>[2x]MGSSHHHHHHSSGLVPRG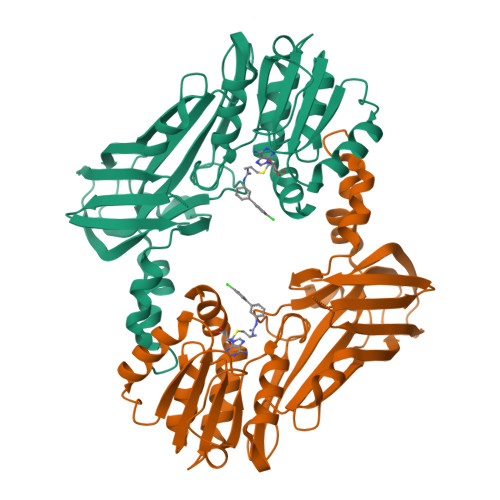SDLQEDEDGVYFSSYGHYGIHEEMLKDKIRTESYRDFIYQNPHIFKDKVVLDVGCGTGILSMFAAKAGAKKVLGVDQSEILYQAMDIIRLNKLEDTITLIKGKIEEVHLPVEKVDVIISEWMGYFLLFESMLDSVLYAKNKYLAKGGSVYPDICTISLVAVSDVNKHADRIAFWDDVYGFKMSCMKKAVIPEAVVEVLDPKTLISEPCGIKHIDCHTTSISDLEFSSDFTLKITRTSMCTAIAGYFDIYFEKNCHNRVVFSTGPQSTKTHWKQTVFLLEKPFSVKAGEALKGKVTVHKNKKDPRSLTVTLTLNNSTQTYGLQ> MADYKDDDDKSGPDEVDASGRMAGMALARAWKQMSWFYYQYLLVTALYMLEPWER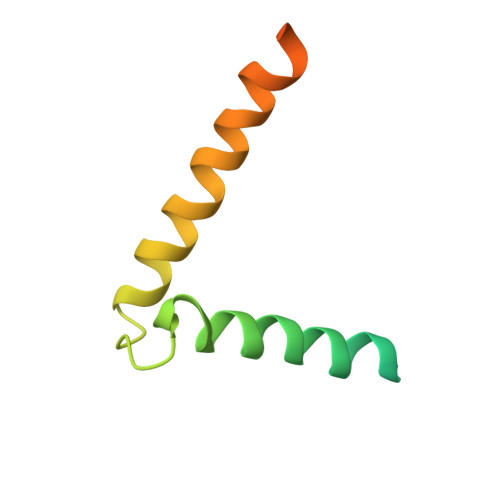TVFNSMLVSIVGMALYTGYVFMPQHIMAILHYFEIVQ>MAHHHHHHMKSIRTLPERKTIALVAHDHKKDDLVRWVQKHAGKLTKHNLIATGTTGKLIEEDLGVEVKRVMSGPLGGDQQLGSMIAQRQIDIVIFFWDPMEAQPHDSDVKAFIRLCVVWNTPMACDSA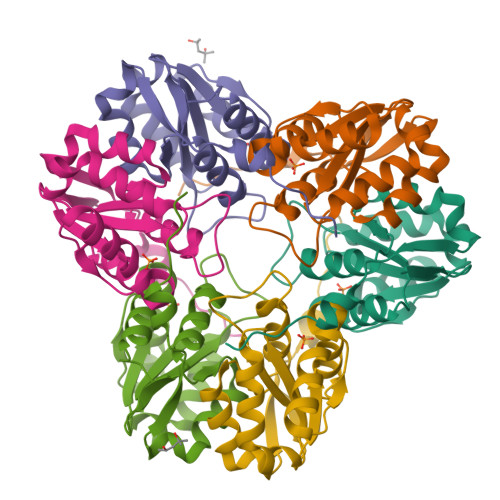TADFILSSPFMETEYQAEIPDYDGYLKRNIPEA[12x]> TTSQKHRDFVAEPMGEKPVGSLAGIGEVLGKKLEERGFDKAYVVLGQFLVLKKDEDL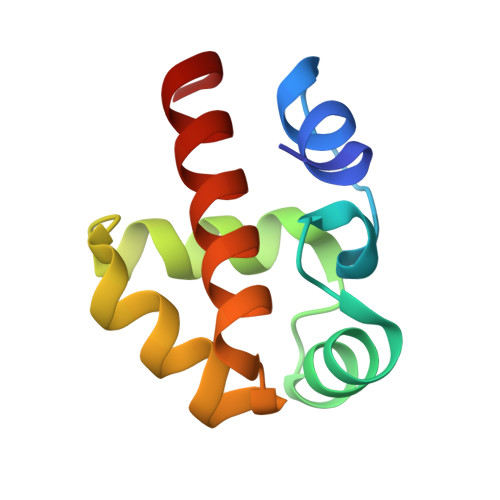FREWLKDTAGANAKQSRDAFGALREWADAFL>[2x]GSMPPQLHNGLDFSAKVIQGSLDSLPQEVRKFVEGNAQLCQPEYIHICDGSEEEYGRLLAHMQEEGVIRKLKKYDNCWLALTDPRDVARIESKTVIITQEQRDTVPIPKSGQSQLGRWMSEEDFEKAFNARFPGCMKGRTMYVIPFSMGPLGSPLAKIGIELTDSPYVVASMRIMTRMGTSVLEALGDGEFIKCLHSVGCPLPLKKPLVNNWACNPELTLIAHLPDRREIISFGSGYGGNSLLGKKCFALRIASRLAKEEGWLAEHM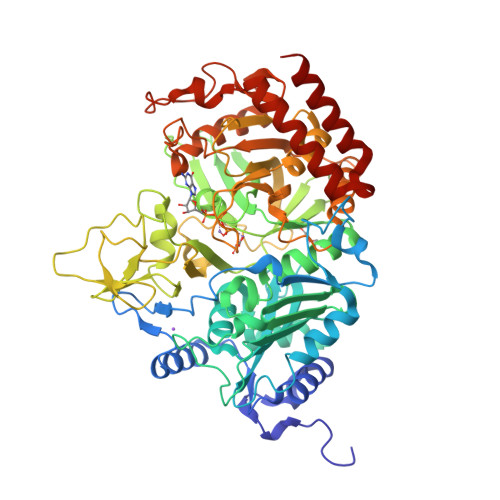LILGITNPEGKKKYLAAAFPSACGKTNLAMMNPTLPGWKVECVGDDIAWMKFDAQGNLRAINPENGFFGVAPGTSVKTNPNAIKTIQKNTIFTNVAETSDGGVYWEGIDEPLAPGVTITSWKNKEWRPQDEEPCAHPNSRFCTPASQCPIIDPAWESPEGVPIEGIIFGGRRPAGVPLVYEALSWQHGVFVGAAMRSEATAAAEHKGKVIMHDPFAMRPFFGYNFGKYLAHWLSMAHRPAAKLPKIFHVNWFRKDKNGKFLWPGFGENSRVLEWMFGRIEGEDSAKLTPIGYVPKEDALNLKGLGDVNVEELFGISKEFWEKEVEEIDKYLEDQVNADLPYEIERELRALKQRISQM>MGSSHHHHHHSSGENLYFQGMNLNKQVAIVTGGASGFGAAIARRLSQAGAAVLVAD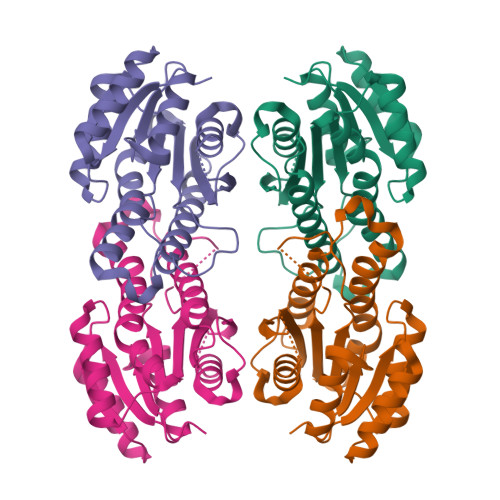LNAEGAQRMATELNAAGGRALGMACDVSKEADYRAVVDAAIAQLGGLHIVVNNAGTTHRNKPALAVTEDEFDRVYRVNLKSVYWSAQCALPHFAQQGHGVMVNVASTTGVRPGPGLTWYSGSKAAMINLTKGLALEFARSGVRINAVNPMIGETPMMADFMGMEDTPANRERFLSRIPLGRFTRPDDVASAVAFLASDDASFLTGVCLDVDGGRNI[2x]> MNNLHRELAPVSDAAWEQIEEEASRTLKRFLAARRVVDVSDPQGPAFSAVGT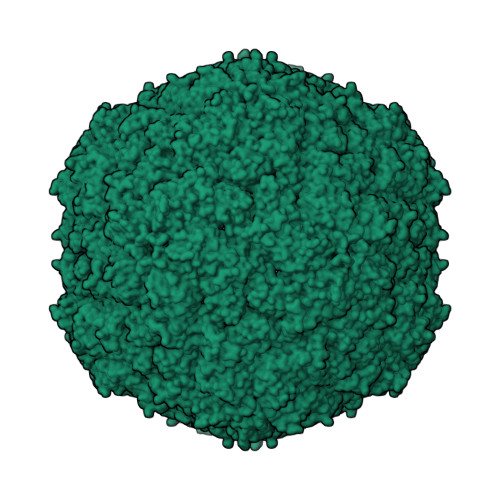GHVTRLEGPGDSVGAVKRQSQPVVEFRVPFILTRQAIDDVERGSQDSDWSPLKEAARKIAGAEDRAVFDGYAAAGIGGIRPQSSNSPLTLPVAASGYPDVIARALDQLRVAGVNGPYHLVLGENAYTLITSGNEDGYPVLQHIHRLIDGEIVWAPAIEGGVLLSTRGGDFAMDIGQDISIGYLSHTATHVELYLQESFTFRTLTSEAVVSLLPSED;> SGSLNIGSLK>STGTFVVSQPLNYRGGARVEPADASGTEKAFEPATGRVIATFTCSGEKEVNLAVQNAKAAFKIWSQKSGMERCRILLEAARIIREREDEIATMECINNGKSIFEARLDIDISWQCLEYYAGLAASMAGEHIQLPGGSFGYTRREPLGVCVGIGAWNYPFQIASWKSAPALACGNAMVFKPSPFTPVSALLLAEIYSEAGVPPGLFNVVQGGAATGQFLCQHPDVAKVSFTGSVPTGMKIMEMSAKGIKPVTLELGGKSPLIIFSDCDMNNAVKGALMANFLTQGQVCCNGTRVFVQKEILDKFTEEVVKQTQRIKIGDPLLEDTRMGPLINRPHLERVLGFVKVAKEQGAKVLCGGDIYVPEDPKLKDGYYMRPCVLTNCRDDMTCVKEEIFGPVMSILSFDTEAEVLERANDTTFGLAAGVFTRDIQRAHRVVAELQAGTCFINNYNVSPVELPFGGYKKSGFGRENGRVTIEYYSQ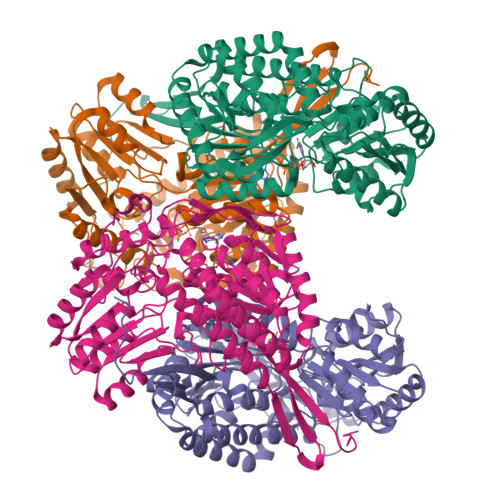LKTVCVEMGDVESAF[8x]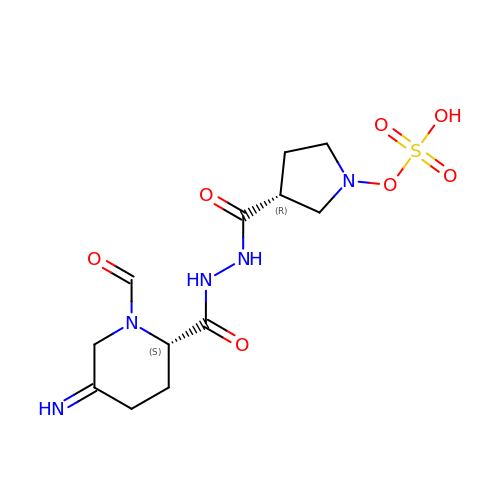(2S,5Z)-1-formyl-5-imino-N'-[(3R)-1-(sulfooxy)pyrrolidine-3-carbonyl]piperidine-2-carbohydrazide | C12 H19 N5 O7 S | APRDZKRWJZJQAT-NBGMFQDKSA-N> DRWGSMTDSEKSATIKVTDASFATDVLSSNKPVLVDFWATWCGPCKMVAPVLEEIATERATDLTVAKLDVDTNPETAR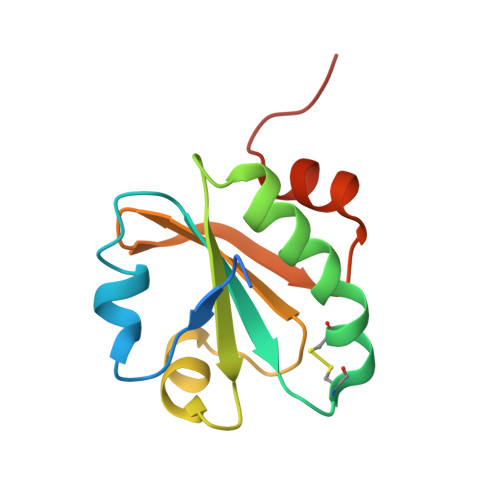NFQVVSIPTLILFKDGQPVKRIVGAKGKAALLRELSDVVPNLN> MNTFGTRLKFTSFGESHGVAVGCIIDGMPAGVKFDEEFLQNELDKRKGGSKFATPRKESDKAQVLSGVFEGYTTGHPIAIVVFNENAHSKDYDNLKDLFRPAHADFTYFYKY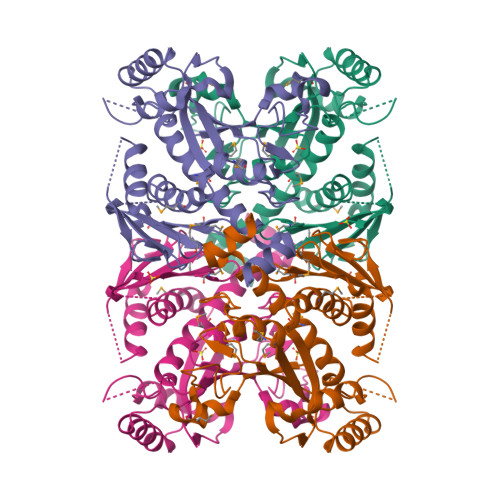GIRDHRGGGRSSARESVARVAGGAVAAMLLREFDICVQSGVFGVGTFVSNLKEEEFDFEFAKKSEIFCLDPKLESDFKNEILNARNSKDSVGAAVFTKVSGMLIGLGEVLYDKLDSKLAHALMGINAVKAVEIGEGINASKMRGSCNNDALKDGKFLSNHSGGILGGISNGENLILKTYFKPTPSIFAKQESIDKFGNNLKFELKGRHDPCVGVRGSVVASAMVRLVLADCLLLNASANLNNLKNAYGLKLEHHHHHH>NAMIIRPEQHWFLRLFDWHGSVLSKIIFRLLLNVLMSIIAIISYQWYEQLGIHLTVAPFSLLGIAIAIFLGFRNS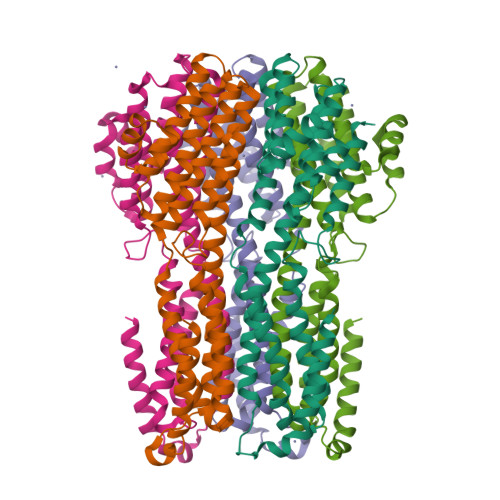ASYSRFVEARNLWGTVLIAERTLVRQLRNILPAEHDAHRRIVSYLVAFSWSLKHQLRKTDPTADLRRLLPEERVTEILASSMPTNRILLLAGNEIGQLREAGKLSDITYGLMDNKLDELAHVLGGCERLATTPVPFAYTLILQRTVYLFCTLLPFALVGDLHYMTPFVSVFISYTFLSFDSLAEELEDPFGTAANDLPLNAMCNTIERNLLDMTGQHPLPE[5x]>MSKKYTQQQYEKYLAQPANNTFGLSPQQVADWFMGQAGARPVINSYGVNASNLVSTYIPKMQEYGVSYTLFLMYTVFEGGGAGNWINHYMYDTGSNGLECLEHDLQYIHGVWETYFPPALSAPECYPATEDNAGALDRFYQSLPGRTWGDVMIPSTMAGNAWVWAYNYCVNNQGAAPLVYFGNPYDSQIDSLLAMGADPFTGGSITGDGKNPSVGTGNATVSASSEANREKLKKALTDLFNNNLEHLSGEFYGNQVLNAMKYGTILKCDLTDDGLNAILQLIADVNLQTNPNPDKPTVQSPGQNDLGSGSDRVAANLANAQAQVGKYIGDGQCYAWVGWWSARVCGYSISYSTGDPMLPLIGDGMNAHSIHLGWDWSIANTGIVNYPVGTVGRKEDLRVGAIWCATAF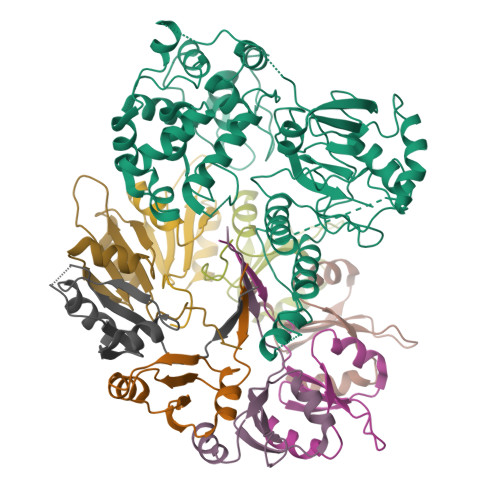SGAPFYTGQYGHTGIIESWSDTTVTVLEQNILGSPVIRSTYDLNTFLSTLTGLITFK[2x];>MSKINVNVENVSGVQGFLFHTDGKESYGYRAFINGVEIGIKDIETVQGFQQIIPSINISKSDVEAIRKAMKK[16x]We show that a nanofluidic sample support with well-defined geometry can be used to prepare cryo-EM specimens with reproducible ice thickness from picoliter sample volumes. The sample solution is contained in electron-transparent nanochannels that provide uniform thickness gradients without further optimisation and eliminate the potentially destructive air-water interface. We demonstrate the performance of this device by high-resolution 3D structure determination of three protein model systems, apoferritin, T20S proteasome, and tobacco mosaic virus. To validate the suitability of cryoChips for 3D structure determination, we collected datasets for three test specimen (P. furiosus ferritin (ApoFtn, 480 kDa, O), T. acidophilum 20 S proteasome (T20S, 700 kDa, D7) and tobacco mosaic virus (TMV, 37 MDa, helical)) that we selected for differences in size, shape and symmetry.

To probe the resolution limit of data collected using the cryoChip, we merged data from three chips filled with ApoFtn acquired on a Titan Krios equipped with a post-GIF K2 camera and processed it in a standard single-particle analysis workflow. We used 2D and 3D classification to select a final set of 21,238 particles (O symmetry) from 815 micrographs and after 3D refinement obtained a reconstruction at an overall resolution of 3.0 Å displaying visible side chain densities (Figure 4c/d). The reference model for 3D alignment was generated from the data itself using the stochastic gradient descent method, suggesting that the quality of data collected from cryoChips is sufficient to allow initial model generation even for samples considered difficult for reference model generation. To examine the compatibility of cryoChips with the condition to form vitreous ice, we evaluated the fraction of images containing crystalline ice by manual inspection for the presence of ice rings or crystalline reflections in the computed power spectra from all images. This led to a fraction of 86% (815/945), 75% (91/121), and 52% (43/82) of images that we classified as containing vitreous ice for ApoFtn, T20S and TMV respectively. For comparison, we also acquired datasets for ApoFtn and T20S on conventional holey carbon supports with the same acquisition parameters, yielding reconstructions at an overall resolution of 2.4 and 3.2 Å. This leads to B-factors of 217 Å2 vs. 178 Å2 for ApoFtn and 490 Å2 vs. 328 Å2 for T20S determined for cryoChip and holey carbon datasets, respectively. Analysis of the orientation distribution showed increased abundance of views along the fourfold rotation axis for ApoFtn, indicating preferential alignment of particles with the SiNx membrane. To quantify this concentration effect, we estimated the particle concentration in the nanochannels by segmenting and counting ApoFtn particles, and measuring the channel volume from the reconstructed tomogram.

> MAMLSERMLKALNDQLNRELYSAYLYFAMAAYFEDLGLEGFANWMKAQAEEEIGHALRFYNYIYDRNGRVELDEIPKPPKEWESPLKAFEAAYEHEKFISKSIYELAALAEEEKDYSTRAFLEWFINEQVEEEASVKKILDKLKFAKDSPQILFMLDKELSARAPKLPGLLMQGGE> GSGMEQFPKETVVESSGPKVLETAEEIQERRQEVLTRYQSFKERVAERGQKLEDSYHLQVFKRDADDLGKWIMEKVNILTDKSYEDPTNIQGKYQKHQSLEAEVQTKSRLMSELEKTREERFTMGHSAHEE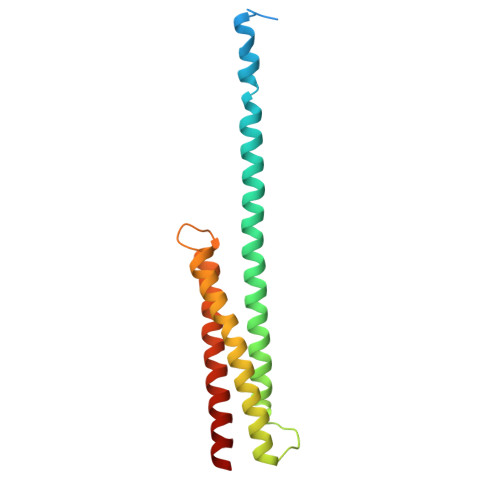TKAHIEELRHLWDLLLELTLEKGDQLLRAL(1R,2S)-N~2~-hydroxy-1-{4-[(2-phenylquinolin-4-yl)methoxy]benzyl}cyclopropane-1,2-dicarboxamide | C28 H25 N3 O4 | 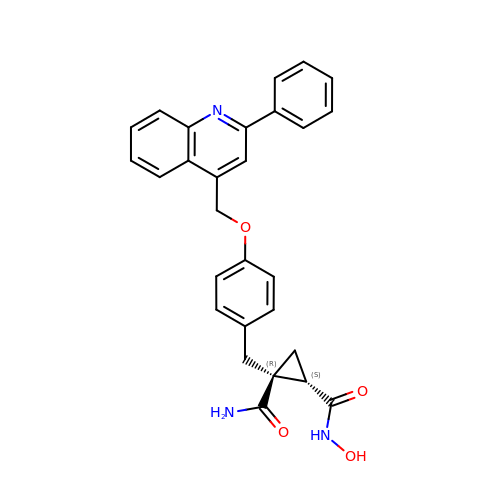BKHGWMSYWJIRLD-LXFBAYGMSA-N> MILWRISAYADLSGTGGLRVSGAWHQAGRPVVY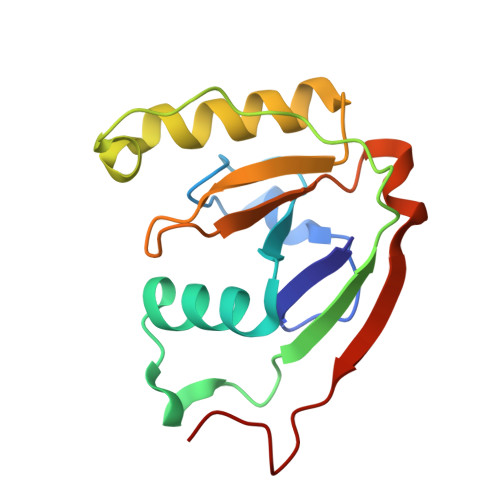AATSPPGAMLEVLVHLEIDPEDFPTTMRLLRIELPDTVSQAQLPALQPGWSAQPELTRTLGNRFLDDCSALLLPVPSAIMPSTTNYLFNPRHPQAQSAKIQVEDFTPDSRLF>MGQAGEITKYVNPFIGTGAIDGGLSGNNYPGATSPFGMIQLSPDTSEAPNWGDASGYDYNRNTIFGFSHTRLSGTGASDLIDITLMPTSSGRTSSAFTHDEEKARPGYYQVMLKDENINAELTTTQRNGIHRYQYPAGKDAEIILDMDHSADKGSWGRRIINSQIRILNDHAVEGYRIITGWAKLRKIYFYMEFSSPILTSTLRDGGRVHENTAVINGTNLHGCFRFGQLNGKPLTCKVALSSVSMENARQNMEQEAPHWDFDRYVAAADADWEKQLGKIEVKGTEVQKEIFYTALYHTMIQPNTMSDVNGEYMAADYTTRKVANNETHYTTFSLWDTFRASHPLYTLLEPERVTDFVKSMIRQYEYYGYLPIWQLWGQDNYCMIGNHSIPVITDAILKGIPGIDMEKAYEAVYNSSVTSHPNSPFEVWEKYGFMPENIQTQSVSITLEQAFDDWCVAQLAAKLNKDADYQRFHKRSEYYRNLFHPKTKFFQSKNDKGEWIEPFDPYQYGGNGGHPFTEGNAWQYFWYVPHNIQALMELTGGTKAFEQKLDTFFTSTYKSEQMNHNASGFVGQYAHGNEPSHHVAYLYNFAGQPWKTQKYVSHILNT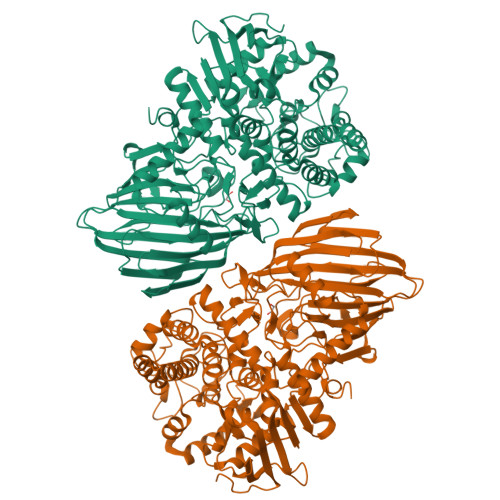LYNNTSSGYAGNDDCGQMSAWYVFSAMGFYPVNPADGRYIIGSPLLDECTLKLAGNKEFRIRTIRKSPEDIYIQSVTLNGKKHKDFFITHQDIMNGGTMVFKMGKKPSGWGKLEHHHHHH[3x]>[2x]MMVLVSYDVSTSSPGGDKRLRKVAKACRDLGQRVQFSVFEIEVDPAQWTALRQRLCDLIDPDIDSLRFYHLGAKWEARVEHVGAKPSLDLKGPLIFLEHHHHHH

Cas2 is a universal Cas protein found in all types of CRISPR-Cas systems, and plays a role in new spacer acquisition during the adaptation stage of CRISPR-Cas immunity. In this study, we describe the structural and functional characterization of Xanthomonas albilineans Cas2 (XaCas2) of a subtype I-C CRISPR-Cas system and provide experimental evidence of pH-dependent conformational switching involving a hinge-bending motion during activation of the dsDNA nuclease function. Overall, the structural features of XaCas2 were similar to those of other subtype I-C Cas2 structures, including the protomer fold, the dimer interface, and the conformational state. The XaCas2 protomer contained an N-terminal ferredoxin fold consisting of a four-stranded antiparallel β-sheet (β1–4) and two α-helices (α1, α2), and a C-terminal segment including a 310-helix (η1) and a β-strand (β5) [Fig. 1(a)]. Although activity was observed under neutral and basic conditions, no dsDNA cleavage was detected at pH 6.0, consistent with the suggestion that the XaCas2 structure crystallized under acidic conditions was in a catalytically inactive conformation. Together, the functional and structural analyses indicate that XaCas2 is a metal- and pH-dependent non-specific dsDNA nuclease, and support the hypothesis that subtype I-C Cas2 proteins undergo a pH-dependent conformational change to allow metal-binding prior to catalysis.

The crystal structures of XaCas2 were determined to resolutions of 1.65 Å and 1.75 Å at 20 and 4 °C, respectively. Data collection and refinement statistics are summarized in Table I. The root mean square deviation (RMSD) of the Cα atomic positions between the two XaCas2 structures was only 0.07 Å, indicating that the two structures were essentially identical. We hereafter describe only the 20 °C structure, which was determined at a higher resolution. The asymmetric unit contained two XaCas2 protomers forming a single dimer with pseudo-two-fold symmetry, 175 water molecules, and three acetate ions. In our crystal structure, XaCas2 seemed to adopt a catalytically inactive conformational state, as was also true of several other subtype I-C Cas2 structures evaluated previously. In the XaCas2 dimer, the two conserved Asp8 residues were too far apart to allow them to coordinate a single catalytic metal ion together [Fig. 1(c)]. The distance between the side chains of the two Asp8 residues was 11.1 Å, and no metal ion was found near the residues. Strikingly, despite the high similarity in overall structure, the two XaCas2 protomers exhibited significant conformational heterogeneity within the putative hinge regions. Without these residues, the RMSD of the Cα atomic positions between the two XaCas2 protomers was only 0.3 Å, whereas the RMSD value for residues 72–78 was 3.5 Å. In protomer A, Lys74 formed salt bridges with Glu40 and interacted hydrophobically with Met2, whereas Trp75 was largely exposed to the solvent.> DPMKNTCKLLVVADHRFYRYMGRGEESTTTNYLIELIDRVDDIYRNTAWDNAGFKGYGIQIEQIRILKSPQEVKPGEKHYNMAKSYPNEEKDAWDVKMLLEQFSFDIAEEASKVCLAHLFTY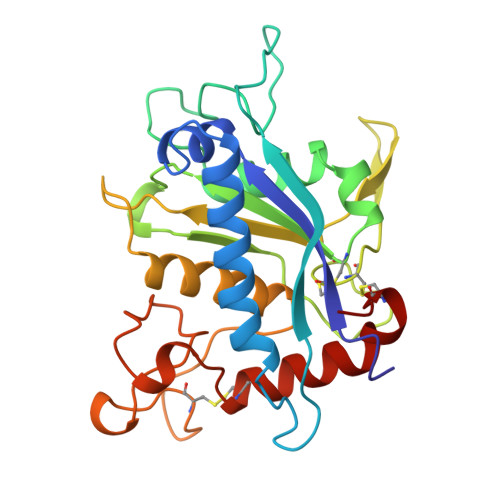QDFDMGTLGLAYVGSPRANSHGGVCPKAYYSPVGKKNIYLNSGLTSTKNYGKTILTKEADLVTTHELGHNFGAEHDPDGLAECAPNEDQGGKYVMYPIAVSGDHENNKMFSQCSKQSIYKTIESKAQECFQERS>MGSEVEILKALLELKKSTAELKRATASLRAITEELKKNPSEDALVEHNRAIVEHNAIIVENNRIIAAVLMLIVVAVGMTQEIKKALEELVASTAELKRATASLRAITEELKKNPSEDALVEHNRAIVEHNAIIVENNRIIAAVLELIVRALNLTDAEVIKALIELRLSTLELVAATASLREITEELKKNPSEDALVEHNRAIVEHN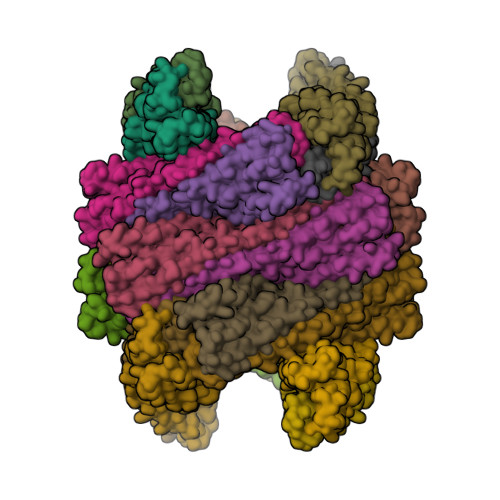AIIVENNRIIAAVLELIVGGSGGSGGSGGSSLEHHHHHH[20x]> MAVTDLSLTNSSLMPTLNPMIQQLALAIAASWQSLPLKPYQLPEDLGYVEGRLEGEKLVIENRCYQTPQFRKMALELAKVGKGLDILHCVMFPEPLYGLPLFGCDIVAGPGGVSAAIADLSPTQSDRQLPAAYQ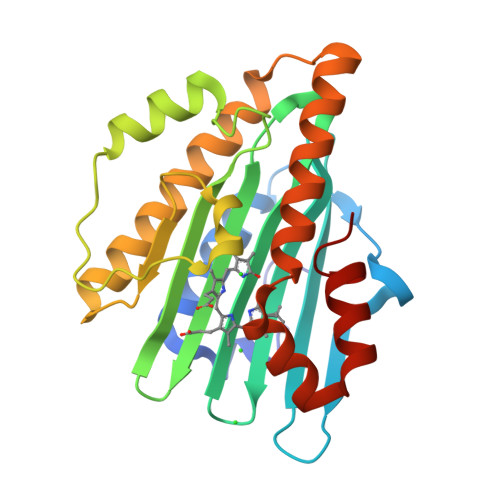KSLAELGQPEFEQQRELPPWGEIFSEYCLFIRPSNVTEEERFVQRVVDFLQIHCHQSIVAEPLSEAQTLEHRQGQIHYCQQQQKNDKTRRVLEKAFGEAWAERYMSQVLFDVIQ1-[2-(4-benzylphenoxy)ethyl]pyrrolidine 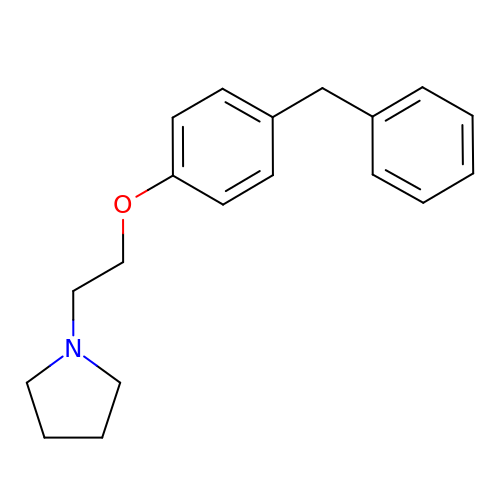| C19 H23 N O | JQTXWEHBUDESJC-UHFFFAOYSA-N> PDQFRAIIESPEGAGHVGYQYRRNTGSTMRMVSDVLDERVSLWDFHCDPSGNVIQPGPNVDSRQYLQAAIDYVSSNGGGTITIPAGYTWYLGSYGVGGIAGHSGIIQLRSNVNLNIEGRIHLSPFFDLKPFQVFVGFDNGDPASSGNLENCHIYGHGVVDFGG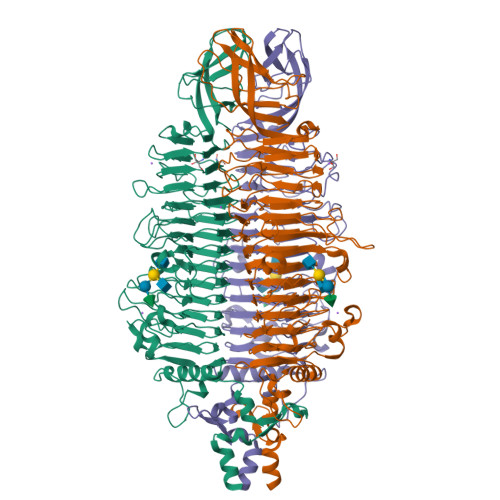YEFGASSQLRNGVAFGRSYNCSVTGITFQNGDVTWAITLGWNGYGSNCYVRKCRFINLVNSSVNADHSTVYVNCPYSGVESCYFSMSSSFARNIACSVALHQHDTFYRGSTVNGYCRGAYVVMHAAEAAGAGSYAYNMQVENNIAVIYGQFVILGSDVTATVSGHLNDVIVSGNIVSIGERAAFSAPFGAFIDIGPDNSGASNVQDIQRVLVTGNSFYAPANITDSAAITLRANLNGCTFIANNFDCRYMVYNAPGTTSPVVQNLVWDKSNVIGGTHANQRAGQNLFDMQFASVVNSTIEVQLSCEDLSMFSCILFPASCQLSYSKITVDSAWTKSMSNTAVFEGNQQAGANVYVSYPATVNLTSYNTQGAVPFFSTDTNYAWVTSAYSLSINENLDFSPPATYTNKANGQLVGVGYNEIGGVRSVSVRLMLQRQV7-(cyclopropylmethyl)-2-methyl-10-[(propan-2-yl)sulfonyl]-2,4,6,7-tetrahydro-3H-2,4,7-triazadibenzo[cd,f]azulen-3-one 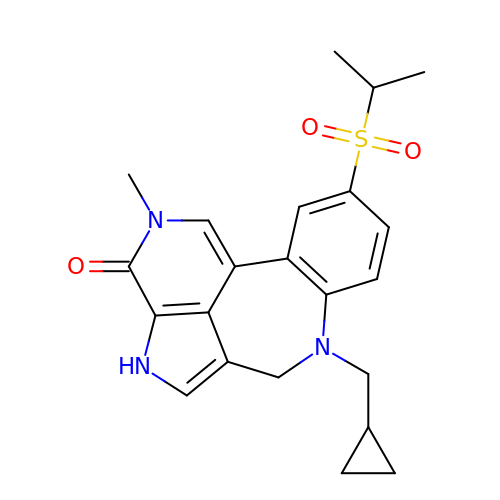| C22 H25 N3 O3 S | AVGPVHNCVRTZSA-UHFFFAOYSA-N>FSCNVDGGSSIGAGTTSVYVNLDPVIQPGQNLVVDLSQHISCWNDYGGWYDTDHINLVQGSAFAGSLQSYKGSLYWNNVTYPFPLTTNTNVLDIGDKTPMPLPLKLYITPVGAAGGVVIKAGEVIARIHMYKIATLGSGNPRNFTWNIISNNSVVMPTGGHHHHHH[2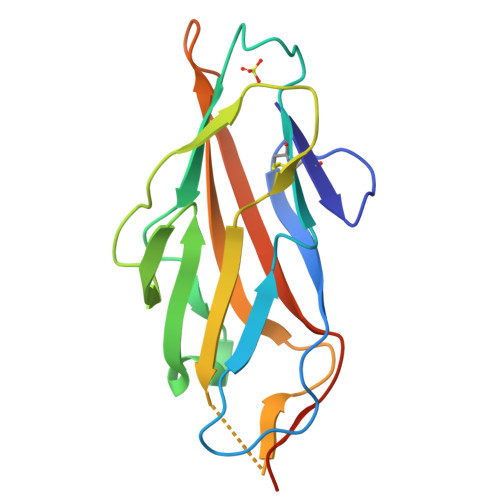x]> SISQQTVWNQMATVRTPLNFDSSKQSFCQFSVDLLGGGISVDKTGDWITLVQNSPISNLLRVAAWKKGCLMVKVVMSGNAAVKRSDWASLVQVFLTNSNSTEHFDACRWTKSEPHSWELIFPIEVCGPNNGFEMWSSEWANQTSWHLSFLVDNPKQSTTFDVLLGISQNFEIAGNTLMPAFSVPQANARSSENAESSA;> METNLFKLSLDDVETPKGSMLDLKISQSKIALPKNTVGGTILRSDLLANFLTEGNFRASVDLQRTHRIKGMIKMVATVGIPENTGIA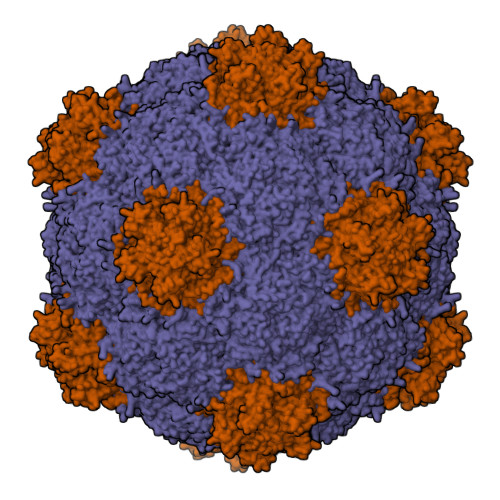LACAMNSSIRGRASSDIYTICSQDCELWNPACTKAMTMSFNPNPCSDAWSLEFLKRTGFHCDIICVTGWTATPMQDVQVTIDWFISSQECVPRTYCVLNPQNPFVLNRWMGKLTFPQGTSRSVKRMPLSIGGGAGAKSAILMNMPNAVLSMWRYFVGDLVFEVSKMTSPYIKCTVSFFIAFGNLADDTINFEAFPHKLVQFGEIQEKVVLKFSQEEFLTAWSTQVRPATTLLADGCPYLYAMVHDSSVSTIPGDFVIGVKLTIIENMCAYGLNPGISGSRLLGTIPQ> LNRLREPLLRRLSELLDQAPEGRGWRRLAELAGSRGRLRLSCLDLEQCSLKVLEPEGSPSLCLLKLMGEKGCTVTELSDFLQAMEHTEVLQL;> EEDLTEVKKDALENLRVYLCEKIIAERHFDHLRAKKILSREDTEEISCRTSSRKRAGKLLDYLQENPKGLDTLVESIRREKTQNFLIQK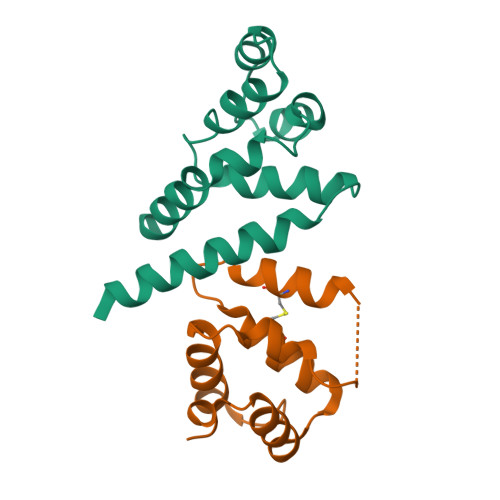ITDEVLKLRNIKLEHLK5'-[2,6-dichloro-4-(propanoylamino)phenoxy]-2'-hydroxybiphenyl-4-carboxamide | C22 H18 Cl2 N2 O4 | 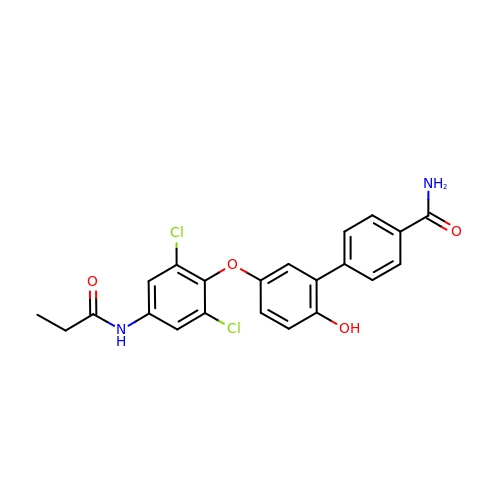PKFMISFXTVJIPA-UHFFFAOYSA-N>[2x]MLKLQTLQALICIEEVGSLRAAAQLLHLSQPALSAAIQQLEDELKAPLLVRTKRGVSLTSFGQAFMKHARLIVTESRRAQEEIGQLRGRWEGHITFAASPAIALAA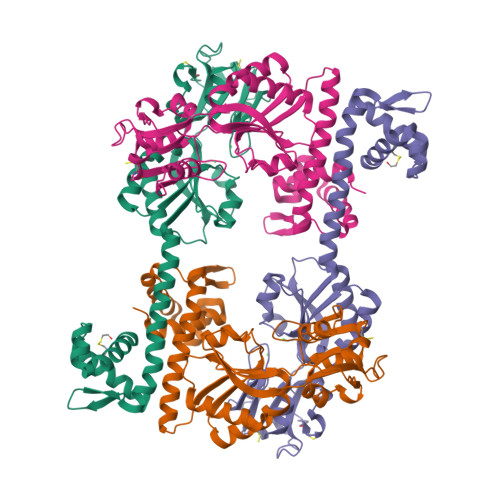LPLALASFAREFPDVTVNVRDGMYPAVSPQLRDGTLDFALTAAHKHDIDTDLEAQPLYVSDVVIVGQRQHPMANATRLAELQECRWAFSSAPRGPGAIIRNAFARYGLPEPKLGLVCESFLALPGVVAHSDLLTTMPRTLYERNAFKDQLCSIPLQDALPNPTIYVLRRHDLPVTPAAAGLIRWIQHHALQTGHHHHHH> MAGTALKRLMAEYKQLTLNPPEGIVAGPMNEENFFEWEALIMGPEDTCFEFGVFPAILSFPLDYPLSPPKMRFTCEMFHPNIYPDGRVCISILHAPGDDPMGYESSAERWSPVQSVEKILLSVVSMLAEPNDESGANVDASKMWRDDREQFYKIAKQIVQKSLGL;> GPSWARQESLQERKQALYEYARRRFTERRAQEAD

Here, we characterize a key role for the UBE2G2 Binding Region (G2BR) of the ERAD accessory protein ancient ubiquitous protein 1 (AUP1) in ERAD pathways. This 27-amino acid (aa) region of AUP1 binds with high specificity and low nanomolar affinity to the backside of the ERAD ubiquitin-conjugating enzyme (E2) UBE2G2. The G2BRAUP1 shares significant structural conservation with the G2BR found in the E3 ubiquitin ligase gp78 and in vitro can similarly allosterically activate ubiquitination in conjunction with ERAD E3s. Thus, by binding to the backside of a critical ERAD E2, G2BRAUP1 plays multiple critical roles in ERAD.

The structure of the AUP1 G2BR (G2BRAUP1) in complex with UBE2G2 reveals an interface that includes a network of salt bridges, hydrogen bonds, and hydrophobic interactions essential for AUP1 function in cells. The UBE2G2:G2BRAUP1 structure reveals UBE2G2 residues 2 to 96 and 107 to 165, G2BRAUP1 residues 377 to 404, and 158 oxygen atoms of water molecules. Residue 1 and residues 97 to 106 of the extended loop characteristic of UBE2G1 and UBE2G2, as well as yeast Ubc7p, are disordered without observable electron density. The overall structure exhibits a high degree of similarity to the previously described structure of UBE2G2:G2BRgp78 with a root–mean–square deviation (RMSD) of 0.5 Å for 167 out of 182 pairs of Cα atoms. The high degree of similarity of the UBE2G2:G2BRAUP1 and UBE2G2:G2BRgp78 structures is the result of a largely conserved set of G2BR residues involved in direct contacts with UBE2G2. Specifically, five positively charged or polar residues of the G2BRAUP1—R382, Q383, K390, R398, and R400—form salt bridges or hydrogen bonds with negatively charged or polar groups on UBE2G2. Mutation of all five of the positively charged or polar G2BRAUP1 residues to glutamate (5E), however, led to a loss of detectable UBE2G2 binding. While the Y394D mutation alone reduced binding, mutation of L386 and Y394 together eliminated detectable binding to UBE2G2. Binding was similarly lost with a single point mutation, A397D, which makes multiple hydrophobic contacts with UBE2G2. The low nanomolar affinity of G2BRAUP1 for UBE2G2 is driven by a combination of salt bridges, hydrogen bonds, and hydrophobic interactions distributed along the length of the UBE2G2:G2BRAUP1 interface as revealed by the crystal structure.1-{3-[7-(difluoromethyl)-6-(1-methyl-1H-pyrazol-4-yl)-3,4-dihydroquinolin-1(2H)-yl]-1-[(3S)-oxolan-3-yl]-1,4,6,7-tetrahydro-5H-pyrazolo[4,3-c]pyridin-5-yl}ethan-1-one | C26 H30 F2 N6 O2 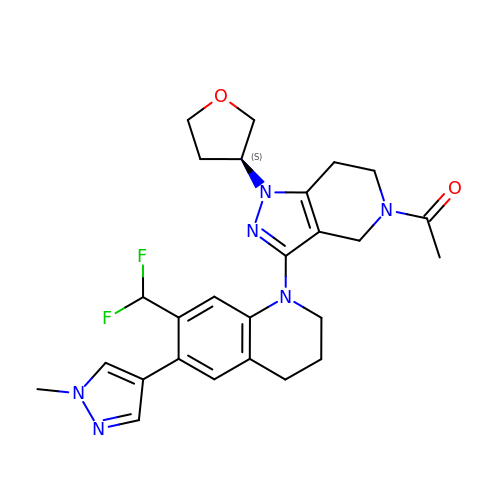| FLTYKXCCCAPRLV-IBGZPJMESA-N>MGSSHHHHHHSSGLVPAGSHMTARATLPYGSWPSPISAADVARARLRLSFPTVAGDDVWWQETRPEEDGRTTVIHLRGGHRTELLQAPWDARTRVHEYGGRSYLPIRTAEGWSVVFSNYDDQRLHRLDEGDPKPYPLTPLPAVPAGLRYADYVLSPDGTEVWCVCEGHIAAPPEPPPAEGEEGAPASEEPAVTGIRRAIVAIPLDGRAAEDAGAIRELVAGAQFYASPAPSPGGGHLAWVQWNHPRMPWDGTEVRVAAVEDGRTVAPRTVKGGLKESALAPLWRDEESLYVISDWPGWWNIYQVGLHGESPQALYPAEEEFAGPLWQLGGMPYALLGDGRLAVLHGEGDLRLGVYDPETLDLVDLEVPYEHWATQLSADGTTVVGIGGGPDLPASVVRVDTTTGRVEGLRRELAELPNVAYLSRPRAERLDGPFGRPVHAYVFPPTNPEAAAPEGELPPYVVFVHGGPTGRVSTVLDLERVYFTSRGIGVIDVNYGGSTGYGRAYRERLRRQWGVVDVEDAIAAAQALVDGGIADPARLAIRGGSAGGWTTLAAITQTDVFKAATSYFGISDLQSFAEATHDFESQYLFGLIGPLPGFERAYEERSPLRHADRTACPVLLLQGLNDPVVPPDQSERFALALADKKMPYAYLTFEGESHGFRKAGTVV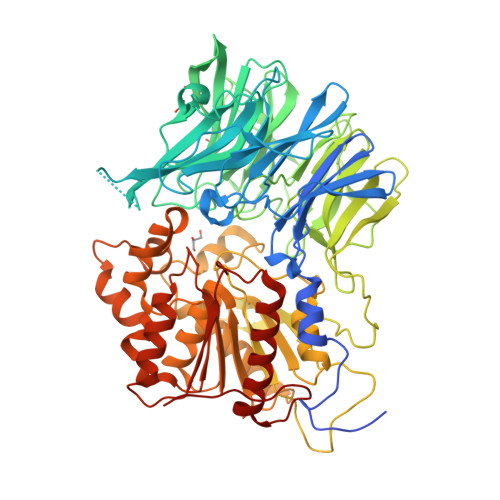RSLEAELAFYGQTLGFEPRGVEPINLTVG[2x]>[2x]MQTEHVILLNAQGVPTGTLEKYAAHTADTRLHLAFSSWLFNAKGQLLVTRRALSKKAWPGVWTNSVCGHPQLGESNEDAVIRRCRYELGVEITPPESIYPDFRFRATDPSGIVENEVCPVF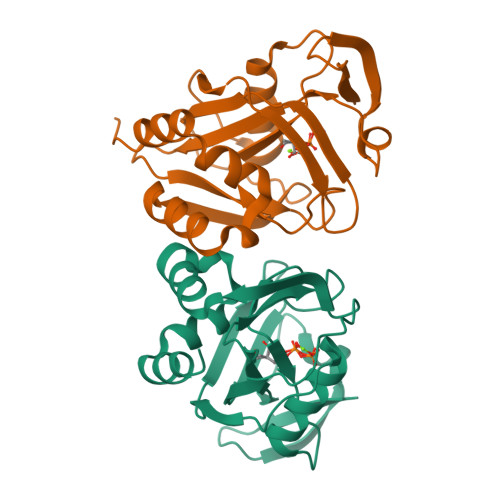AARTTSALQINDDEVMDYQWCDLADVLHGIDATPWAFSPWMVMQATNREARKRLSAFTQLKL>YIDTN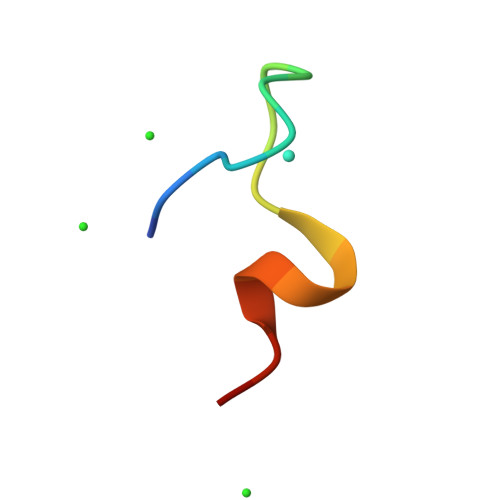NDGWYEGDELLAX[2x]>[2x]SNAMDRIVEIEKYSFDETYETSLRPSNFDGYIGQESIKKNLNVFIAAAKKRNECLDHILFSGPAGLGKTTLANIISYEMSANIKTTAAPMIEKSGDLAAILTNLSEGDILFIDEIHRLSPAIEEVLYPAMEDYRLDIIIGS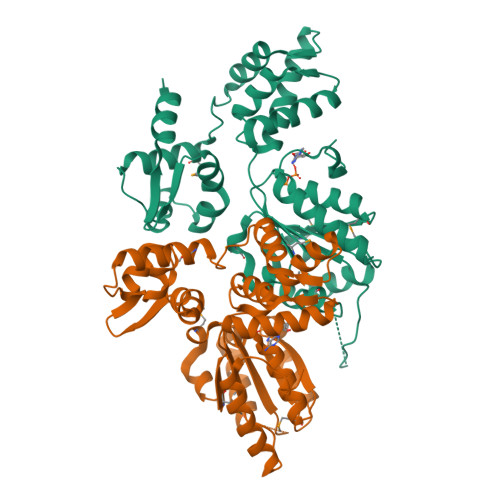GPAAQTIKIDLPKFTLIGATTRAGMLSNPLRDRFGMQFRLEFYKDSELALILQKAALKLNKTCEEKAALEIAKRSRSTPRIALRLLKRVRDFADVNDEEIITEKRANEALNSLGVNELGFDAMDLRYLELLTAAKQKPIGLASIAAALSEDENTIEDVIEPYLLANGYIERTAKGRIASAKSYSALKLNYEKTLFEE>[2x]MIFTNAILVISALLPATVLSLQHTEDSLFPARCWPDPCAGITFQNDTYVCGDPRLGPVVLPQKFPLNNELRTYARFGALCPAEFLDKWATDVAPNGTYIYPPANG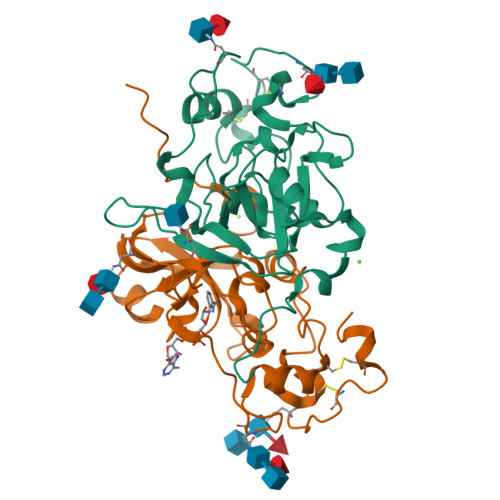FALDTEEQPILGNATLPVGMKLDRFGSEYGTFLAPLGAPYIERSLPPSNLNTFDGMYPYNYHVYQVTKEFVVGLGPIAPWFEQPGMGTQFVTYTNVLGLIDDGYLRRLDESEYDEKVEYSNPYTPGPNQDVLFQGPGHHHHHH> MHHHHHHSSGLEVLFQGPGSPYFHSFLYMNGGLMNSWKRRWCVLKDETFLWFRSKQEALKQGWLHNNGGGSSTLSRRNWKKRWFVLRQSKLMYFENDSEEKLKGTVEVRSAKEIIDNTNKENGIDIIMADRTFHLIAESPEDASQWFSVLSQVHSSTDQEIREMHDEQANPQNAVGTLDVGLIDSVCASDSPDRPNSFVIITA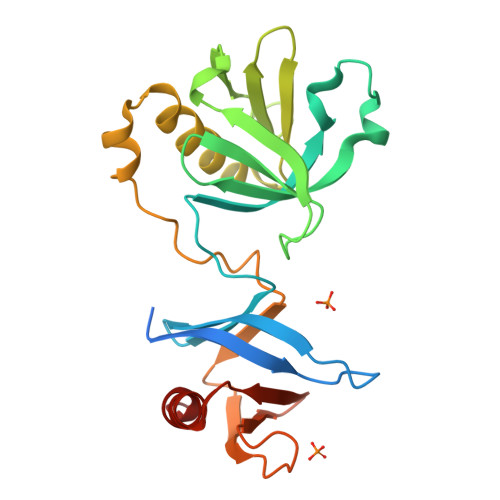NRVLHCNADTPEEMHHWITLLQRSK>SVTEFLKPRLVDIEQVSSTHAKVTLEPLERGFGHTLGNALRRILLSSMPGCAVTEVEIDGVLHEYSTKEGVQEDILEILLNLKGLAVRVQGKDEVILTLNKSGIGPVTAADITHDGDVEIVKPQHVICHLTDENASISMRIKVQRGRGYVPASTRIHSEEDERPIGRLLVDACYSPVERIAYNVEAARVEQRTDLDKLVIEMETNGTIDPEEAIRRAATILAEQLEAFVDLRDVRQPEVKEEKPEFDPILLRPVDDLELTVRSANCLKAEAIHYIGDLVQRTEVELLKTPNLGKKSLTEIKDVLASRGLSLGMRLENWPPA[2x];> MVYSYTEKKRIRKDFGKRPQVLDVPYLLSIQLDSFQKFIEQDPEGQYGLEAAFRSVFPIQSYSGNSELQYVSYRLGEPVFDVQECQIRGVTYSAPLRVKLRLVIYEREAPEGTVKDIKEQEVYMGEIPLMTDNGTFVINGTERVIVSQLHRSPGVFFDSDKGKTHSSGKVLYNARIIPYRGSWLDFEFDPKDNLFVRIDRRRKLPATIILRALNYTTEQILDLFFEKVIFEIRDNKLQMELVPERLRGETASFDIEANGKVYVEKGRRITARHIRQLEKDDVKLIEVPVEYIAGKVVAKDYIDESTGELICAANMELSLDLLAKLSQSGHKRIETLFTNDLDHGPYISETLRVDPTNDRLSALVEIYRMMRPGEPPTREAAESLFENLFFSEDRYDLSAVGRMKFNRSLLREEIEGSGILSKDDIIDVMKKLIDIRNGKGEVDDIDHLGNRRIRSVGEMAENQFRVGLVRVERAVKERLSLGDLDTLMPQDMINAKPISAAVKEFFGSSQLSQFMDQNNPLSEITHKRRISALGPGGLTRERAGFEVRDVHPTHYGRVCPIETPEGPNIGLINSLSVYAQTNEYGFLETPYRKVTDGVVTDEIHYLSAIEEGNYVIAQANSNLDEEGHFVEDLVTCRSKGESSLFSRDQVDYMDVSTQQVVSVGASLIPFLEHDDANRALMGANMQRQAVPTLRADKPLVGTGMERAVAVDSGVTAVAKRGGVVQYVDASRIVIKVNEDEMYPGEAGIDIYNLTKYTRSNQNTCINQMPCVSLGEPVERGDVLADGPSTDLGELALGQNMRVAFMPWNGYNFEDSILVSERVVQEDRFTTIHIQELACVSRDTKLGPEEITADIPNVGEAALSKLDESGIVYIGAEVTGGDILVGKVTPKGETQLTPEEKLLRAIFGEKASDVKDSSLRVPNGVSGTVIDVQVFTRDGVEKDKRALEIEEMQLKQAKKDLSEELQILEAGLFSRIRAVLVAGGVEAEKLDKLPRDRWLELGLTDEEKQNQLEQLAEQYDELKHEFEKKLEAKRRKITQGDDLAPGVLKIVKVYLAVKRRIQPGDKMAGRHGNKGVISKINPIEDMPYDENGTPVDIVLNPLGVPSRMNIGQILETHLGMAAKGIGDKINAMLKQQQEVAKLREFIQRAYDLGADVRQKVDLSTFSDEEVMRLAENLRKGMPIATPVFDGAKEAEIKELLKLGDLPTSGQIRLYDGRTGEQFERPVTVGYMYMLKLNHLVDDKMHARSTGSYSLVTQQPLGGKAQFGGQRFGEMEVWALEAYGAAYTLQEMLTVKSDDVNGRTKMYKNIVDGNHQMEPGMPESFNVLLKEIRSLGINIELED;> LLKFLKAQTKTEEFDAIKIALASPDMIRSWSFGEVKKPETINYRTFKPERDGLFCARIFGPVKDYECLCGKYKRLKHRGVICEKCGVEVTQTKVRRERMGHIELASPTAHIWFLKSLPSRIGLLLDMPLRDIERVLYFESYVVIEGGMTNLERQQILTEEQYLDALEEFGDEFDAKMGAEAIQALLKSMDLEQECEQLREELNETNSETKRKKLTKRIKLLEAFVQSGNKPEWMILTVLPVLPPDLRPLVPLDGGRFATSDLNDLYRRVINRNNRLKRLLDLAAPDIIVRNEKRMLQEAVDALLDNGRRGRAITGSNKRPLKSLADMIKGKQGRFRQNLLGKRVDYSGRSVITVGPYLRLHQCGLPKKMALELFKPFIYGKLELRGLATTIKAAKKMVEREEAVVWDILDEVIREHPVLLNRAPTLHRLGIQAFEPVLIEGKAIQLHPLVCAAYNADFDGDQMAVHVPLTLEAQLEARALMMSTNNILSPANGEPIIVPSQDVVLGLYYMTRDCVNAKGEGMVLTGPKEAERLYRSGLASLHARVKVRITEYEKDANGELVAKTSLKDTTVGRAILWMIVPKGLPYSIVNQALGKKAISKMLNTCYRILGLKPTVIFADQIMYTGFAYAARSGASVGIDDMVIPEKKHEIISEAEAEVAEIQEQFQSGLVTAGERYNKVIDIWAAANDRVSKAMMDNLQTETVINRDGQEEKQVSFNSIYMMADSGARGSAAQIRQLAGMRGLMAKPDGSIIETPITANFREGLNVLQYFISTHGARKGLADTALKTANSGYLTRRLVDVAQDLVVTEDDCGTHEGIMMTPVIEGGDVKEPLRDRVLGRVTAEDVLKPGTADILVPRNTLLHEQWCDLLEENSVDAVKVRSVVSCDTDFGVCAHCYGRDLARGHIINKGEAIGVIAAQSIGEPGTQLTMRTFHIGGAASRAAAESSIQVKNKGSIKLSNVKSVVNSSGKLVITSRNTELKLIDEFGRTKESYKVPYGAVLAKGDGEQVAGGETVANWDPHTMPVITEVSGFVRFTDMIDGQTITRQTDELTGLSSLVVLDSAERTAGGKDLRPALKIVDAQGNDVLIPGTDMPAQYFLPGKAIVQLEDGVQISSGDTLARIPQESGGTKDITGGLPRVADLFEARRPKEPAILAEISGIVSFGKETKGKRRLVITPVDGSDPYEEMIPKWRQLNVFEGERVERGDVISDGPEAPHDILRLRGVHAVTRYIVNEVQDVYRLQGVKINDKHIEVIVRQMLRKATIVNAGSSDFLEGEQVEYSRVKIANRELEANGKVGATYSRDLLGITKASLATESFISAASFQETTRVLTEAAVAGKRDELRGLKENVIVGRLIPAGTGYAYHQDRMRRRAAG;> ARVTVQDAVEKIGNRFDLVLVAARRARQMQVGGKDPLVPEENDKTTVIALREIEEGLINNQILDVRERQEQQEQ;> TAGTPSGNGVDYQDDELPVYQGETTQSLQDYLMWQVELTPFTDTDRAIATSIVDAVDDTGYLTIQIEDIVDSIGDDEIGLEEVEAVLKRIQRFDPVGVAAKDLRDCLLIQLSQFAKETPWLEEARLIISDHLDLLANHDFRTLMRVTRLKEEVLKEAVNLIQSLDPRPGQSIQTGEPEYVIPDVLVRKVNDRWVVELNSDSLPRLKINQQYAAMGNSARNDADGQFIRSNLQEARWLIKSLESANDTLLRVSRCIVEQQQAFFEQGEEYMKPMVLADIAQAVEMHESTISRVTTQKYLHSPRGIFELKYFFSSHVNTEGGGEASSTAIRALVKKLIAAENPAKPLSDSKLTSMLSEQGIMVARRTVAKYRESLSIPPSNQ

Transcription initiation in bacteria involves the recruitment of RNAP by sigma factors (σ) to promoter regions located upstream from the transcription start site (TSS, position +1). In approximately 60% of bacteria, a major variant σ factor, σ54, forms a class of its own, lacking structural and sequence similarity to σ70. In σ54-mediated transcription initiation, σ54 recruits RNAP to genes responsible for regulating a variety of stress responses, including nutrient depletion, membrane stress, antibiotic exposure, and biofilm formation. In this study, we used single-particle cryo-electron microscopy (cryoEM) to determine the structures of initial transcribing complexes of increasing RNA lengths from 5 nt to 9 nt, which allow us to propose a mechanism of RNAP promoter escape in the σ54 system.

Using a combination of focused classification and electron density subtraction, we obtained several distinct structural states within the same dataset, including pre- and post-translocated RNA states, as well as σ-free states. We focused on the pre- and post-translocated states which were resolved to 2.8 and 3.4 Å resolution respectively based on gold standard Fourier Shell Correlation curves. We could resolve almost the entire RNAP (including one α-CTD), DNA between −29 and +20, 5 nt RNA as well as σ54 CBD, ELH-HTH, and RpoN domains. In the RPitc-5nt structures, we could resolve extra residues in RII, including 93–106 (Inset). In RPitc-5nt, residues 104–112 form the tip of a β-hairpin (Inset), and residues 93–103 emerge from the β subunit side of the RNAP instead (Left). We now refer to this β-hairpin (residues 104–112) as the RII-finger due to its functional similarity with the σ70 finger, also known as R3.2 in σ70. In RPitc-5nt, RII contacts the template strand at the −5 position, and threads around the template DNA–RNA hybrid and forms a sharp kink at P110 (Inset). The RII-finger is stabilized by hydrophobic interactions between P110 and Y112 of RII, and the conserved P251, V253, and P254 on the β′ lid and M330 on β′ switch 2 region (Inset). During initial transcription, as in RPitc-5nt, the template strand expands into the back of the cleft. The template strand now interacts with the σ54 RII-finger.> MSPPTASASVASSGSSPHMDRLLGDLKLLAAYDSAAGWQEPKAMESAFQSLSWDDADVLKALPQYLNCRGEQKRRVDFA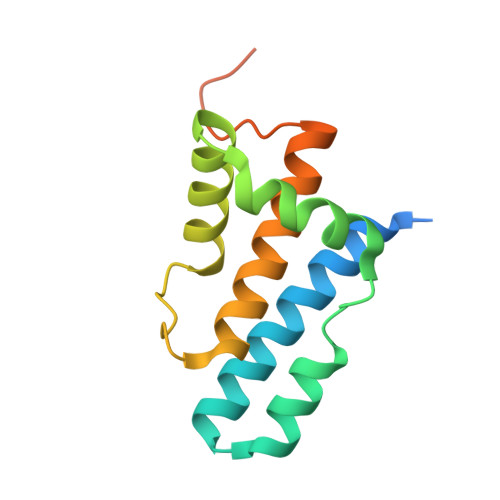YAALCPRPVDEKDPKQTLMSLWMKARLFSYDQKHPFVLSPFAATDKSTSAGAMTAEKPF>[6x]MQRASRLKRELHMLATEPPPGITCWQDKDQMDDLRAQILGGANTPYEKGVFKLEVIIPERYP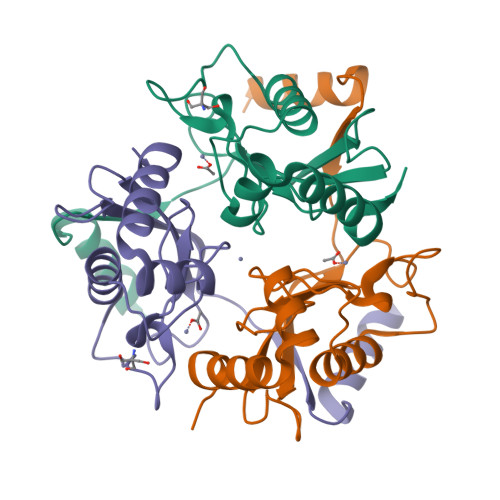FEPPQIRFLTPIYHPNIDSAGRICLDVLKLPPKGAWRPSLNIATVLTSIQLLMSEPNPDDPLMADISSEFKYNKPAFLKNARQWTEKHARQK>[2x]MARIRARGSSRVDVPKENTTAQNKFTSQASDK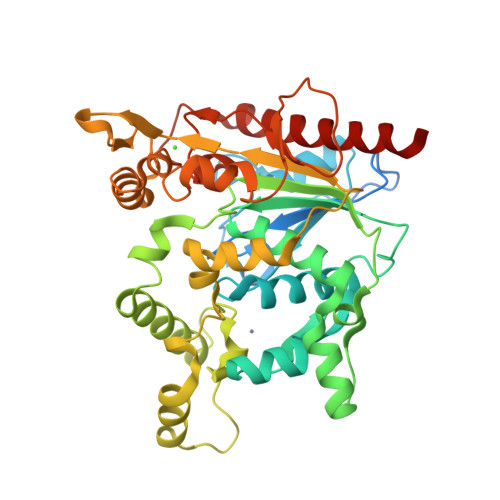KPTVKAAPEAVQNPENPKNKDPFVFVHGFTGFVGEVAAKGENYWGGTKANLRNHLRKAGYETYEASVSALASNHERAVELYYYLKGGRVDYGAAHSEKYGHERYGKTYEGVLKDWKPGHPVHFIGHSMGGQTIRLLEHYLRFGDKAEIAYQQQHGGIISELFKGGQDNMVTSITTIATPHNGTHASDDIGNTPTIRNILYSFAQMSSHLGTIDFGMDHWGFKRKDGESLTDYNKRIAESKIWDSEDTGLYDLTREGAEKINQKTELNPNIYYKTYTGVATHETQLGKHIADLGMEFTKILTGNYIGSVDDILWRPNDGLVSEISSQHPSDEKNISVDENSELHKGTWQVMPTMKGWDHSDFIGNDALDTKHSAIELTNFYHSISDYLMRIEKAESTKNA> MVKVLFFAQVRELVGTDATEVAADFPTVEALRQHMAAQSDRWALALEDGKLLAAVNQTLVSFDHPLTDGDEVAFFPPVTGG;> MAETKIVVGPQPFS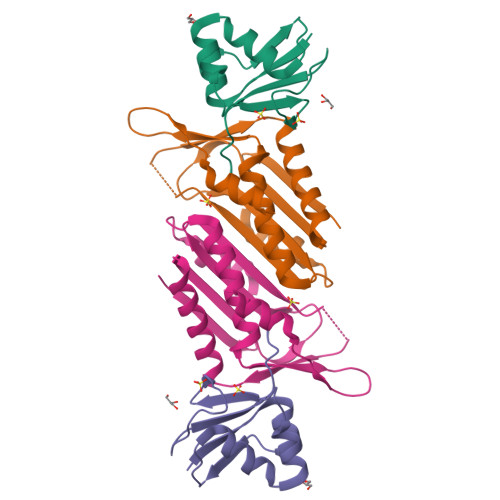VGEEYPWLAERDEDGAVVTFTGKVRNHNLGDSVNALTLEHYPGMTEKALAEIVDEARNRWPLGRVTVIHRIGELWPGDEIVFVGVTSAHRSSAFEAGQFIMDYLKTRAPFWKREATPEGDRWVEARESDQQAAKRW> MKISVSKNDLENALRYLQAFLDKKDASSIASHIHLEVIKEKLFLKASDSDIGLKSYIFTQSSDKEGVGTINGKKFLDIISCLKDSNIILETKDDSLAIKQNKSSFKLPMFDADEFPEFPVIDPKVSIEVNAPFLVDAFKKIAPVIEQTSHKRELAGILMQFDQKHQTLSVVGTDTKRLSYTQLEKISIHSTEEDISCILPKRALLEILKLFYENFSFKSDGMLAVIENEMHTFFTKLIDGNYPDYQKILPKEYISSFTLGKEEFKESIKLCSSLSSTIKLTLEKNNALFESLDSEHSETAKTSVEIEKGLDIEKAFHLGVNAKFFLEALNALGT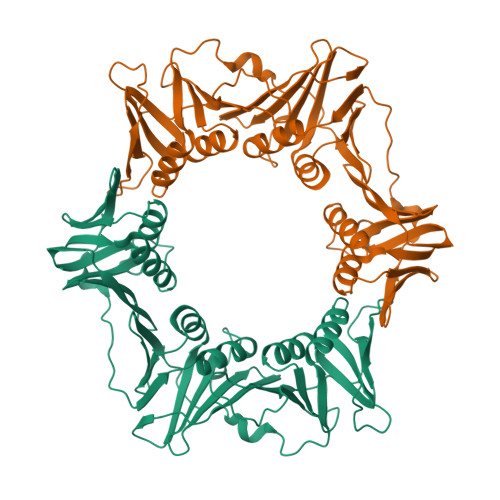TQFVLRCNEPSSPFLIQESLDEKQSHLNAKISTLMMPITLLEHHHHHH>MANVSKKVSWSGRDRDDEEAAPLLRRTARPGGGTPLLNGAGPGAARQSPRSALFRVGHMSSVELDDELLDPDMDPPHPFPKEIPHNEKLLSLKYESLDYDNSENQLFLEEERRINHTAFRTVEIKRWVICALIGILTGLVACFIDIVVENLAGLKYRVIKGNIDKFTEKGGLSFSLLLWATLNAAFVLVGSVIVAFIEPVAAGSGIPQIKCFLNGVKIPHVVRLKTLVIKVSGVILSVVGGLAVGKEGPMIHSGSVIAAGISQGRSTSLKRDFKIFEYFRRDTEKRDFVSAGAAAGVSAAFGAPVGGVLFSLEEGASFWNQFLTWRIFFASMISTFTLNFVLSIYHGNMWDLSSPGLINFGRFDSEKMAYTIHEIPVFIAMGVVGGVLGAVFNALNYWLTMFRIRYIHRPCLQVIEAVLVAAVTATVAFVLIYSSRDCQPLQGGSMSYPLQLFCADGEYNSMAAAFFNTPEKSVVSLFHDPPGSYNPLTLGLFTLVYFFLACWTYGLTVSAGVFIPSLLIGAAWGRLFGISLSYLTGAAIWADPGKYALMGAAAQLGGIVRMTLSLTVIMMEATSNVTYGFPIMLVLMTAKIVGDVFIEGLYDMHIQLQSVPFLHWEAPVTSHSLTAREVMSTPVTCLRRREKVGVIVDVLSDTASNHNGFPVVEHADDTQPARLQGLILRSQLIVLLKHKVFVERSNLGLVQRRLRLKDFRDAYPRFPPIQSIHVSQDERECTMDLSEFMNPSPYTVPQEASLPRVFKLFRALGLRHLVVVDNRNQVVGLVTRKDLARYRLGKRGLEELSLAQT[2x];>[2x]MEPGPTAAQRRCSLPPWLPLGLLLWSGLALGALPFGSSPHRVFHDLLSEQQLLEVEDLSLSLLQGGGLGPLSLPPDLPDLDPECRELLLDFANSSAELTGCLVRSARPVRLCQTCYPLFQQVVSKMDNISRAAGNTSESQSCARSLLMADRMQIVVILSEFFNTTWQEANCANCLTNNSEELSNSTVYFLNLFNHTLTCFEHNLQGNAHSLLQTKNYSEVCKNCREAYKTLSSLYSEMQKMNELENKAEPGTHLCIDVEDAMNITRKLWSRTFNCSVPCSDTVPVIAVSVFILFLPVVFYLSSFLHSEQKKRKLILPKRLKSSTSFANIQENSN

Lysosomes process cellular waste and coordinate responses to metabolic challenge. Central to lysosomal homeostasis are phosphoinositide lipids, key signaling molecules which establish organelle identity, regulate membrane dynamics and are tightly linked to the pathophysiology and therapy of lysosomal storage disorders, neurodegeneration, and cancer. Phosphatidylinositol 3,5- bisphosphate (PI(3,5)P2) interacts with multiple lysosomal membrane proteins and plays a critical role in regulating lysosomal pH by directly inhibiting the chloride/proton antiporter ClC-7, though the molecular mechanism of this inhibition remains unclear.

Here, using a combination of functional, structural, and computational analysis, we demonstrate that PI(3,5)P2 binding dramatically remodels the structure of ClC-7 by inducing close association between cytosolic and transmembrane domains. Conversely, ClC-7 activation is correlated with dissociation and increased disorder of the cytoplasmic domain along with novel transmembrane domain conformations, revealing a mechanistic link between specific lysosomal lipids, transporter regulation, and the enigmatic basis of the ClC-7 slow gate.6-{4-[3-(dimethylamino)propoxy]phenyl}-2-(methylsulfonyl)-N-[3-(1H-pyrazol-1-yl)propyl]pyrimidin-4-amine | C22 H30 N6 O3 S | 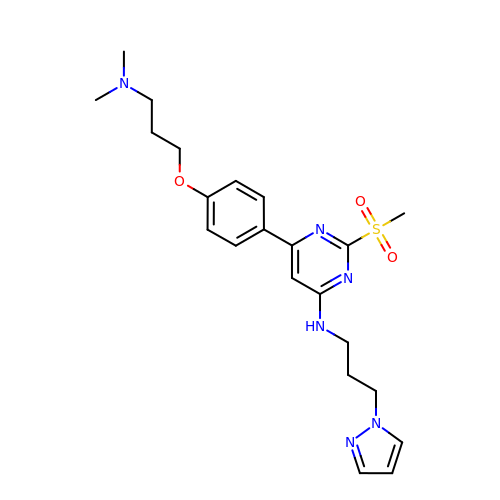MSIJJXOWLFOYIN-UHFFFAOYSA-N>[2x]HMSAADFEAAVAYVRSLPKDGPVQL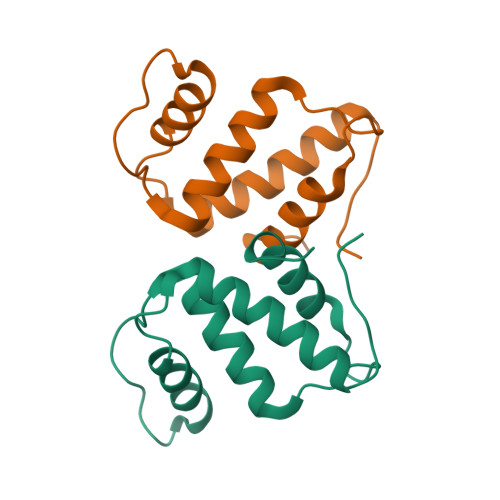DNAAKLQFYSLYKQATEGDVTGSQPWAVQVEARAKWDAWNSCKGMKSEDAKAAYVRRLLTLLRSQGIQWKPGGARVQSR>SNAMHIRDMLAEAERTGEPSFSFQYFPPKTAQGVQNLYDRMERMYNYGPKFIDITWGAGGRVAELTCEMVVQAQAYLGLETCMHLTCTDMGVERINDALRKAYKAGCTNILALRGDPPRDKEKWEAAKDGFRYAKDLVAHIRKEYGDHFDIGVAGYPEGCDDNKDEDLLLDHLKEKVDMGAGFIVTQMFYDVDNFLRWVKKVRERGISVPIVPGIMPIATYASFLRRANHMKCKIPEEWMAKLEPVKNDDVAVREIGKTLVADMCRKILDAGIRHLHFYTMNLAQATRMVLEELNWLPSPDRPLKHALPWKQSLGFGRRGEDVRPIFWRNRNKSYVARTQDWDEFPNGRWGDSRSPAFGELDAYGVGLTGSNEQNRERWGEPKCIRDIANLFIRYMRKEIDYLPWSEAPVADEADLIKDELIDLNRRGLITVNSQPAVNGAKSNHPVHGWGPSNGYVYQKAYLEFFVSPELYPEIKRRIESHPDLTYHAVTKSGNLETNAQSDGPNAVTWGVFPGKEIFQPTIVERISFLAWKDEAYHLGMEWARCYDAGSPSRVLLEEMMNTWWLVNIVNNDFHQGNTLFEILKGLEVTDLDKVPETQANGTNGVSNGVKASETSV[4x]

Methylenetetrahydrofolate reductase (MTHFR) is a pivotal flavoprotein connecting the folate and methionine methyl cycles, catalyzing the conversion of methylenetetrahydrofolate to methyltetrahydrofolate. The eukaryotic form of MTHFR is homodimeric, where each monomer consists of the N-terminal catalytic domain connected by a linker to the C-terminal regulatory domain. In addition, AdoMet acts as an allosteric regulator of MTHFR and a feedback loop regulator in folate and methionine metabolism. Here, we report crystal structures of Chaetomium thermophilum MTHFR (cMTHFR) in both active (R) and inhibited (T) states.

As such, a mutant (cMTHFRE21Q, L393M, V516F) was used instead, along with reductive methylation of surface-exposed lysine residues to aid in crystallization. The construct was successfully crystallized, and its structure was solved to 3.4 Å in the active R-state. Electron density for FAD was observed in every catalytic active site. Although electron density consistent with AdoHcy was found in the regulatory domain, it was weak and could not be faithfully modeled. Even so, the homodimer assembly was found to display the same dimer interface mediated by the regulatory domain, a β-sheet sandwich consistent with the one previously observed for AdoHcy-bound hMTHFR (R-state)7. The catalytic domains were also found to face “away” from the dimer interface and each other and are not interacting with one another, in stark contrast to the direct role they play in dimerization in bacterial MTHFRs. In this active R-state, the si-face of FAD is unoccluded in the active site and forms an extended hydrogen-bonding network between N5 of FAD centered on conserved residues His81 and Asp50 (His127 and Asp92 in hMTHFR), along with a strong hydrogen bond between the universally conserved Thr52 (Thr94 in hMTHFR) and O4 of FAD. Given that the active site is solvent exposed and that access to FAD is unoccluded, the captured structure likely represents a catalytically-competent form of the enzyme in the active R-state, much like that observed for hMTHFR. When the linker between the catalytic and regulatory domains is retracted, Arg315 can interact with Glu318 and Thr336 in this active state.>MQARARAFRLKSYADGDLLRELRQFDGAKNASELGPRAFVRDSHRLDAAVEKASKLTDPTFHISQYQLPHPYSFGGGPPNPERPLTAPLISAINKVSQRTRDPVGYRKRAKESIDLGDFTTHDPDTLHPRFLEYVHERTRSVDGPTDDAMRAAQTVFARLWRRKGCKVKARSLSDAQPDNLLAIIKKGSPGEYRSLGAEDRRDPRLIATMSSSLLRYASAGVQVARGRPPPGWVDTTTQVTLTFGKREPKAAKIVDGVRQAPVPRFIFNLSPVNYALASFLHYDISHFLMDNDPTHGPGFGPGRGRARKFMDLVERAFDGRFSTPDGARLIMSDITKWDANMCEALIKYSIDLLEDAVDKSALSPEGLATRGLMYRVARRQLLEKLVEHPAGYFVKLYGCMPSGSFYTSLVNTTGNNLLVIGHAIARAVEETSLTHHGAAELLADAVDGTLISYGDNQLFSEHLFSVLGLAYDPEKH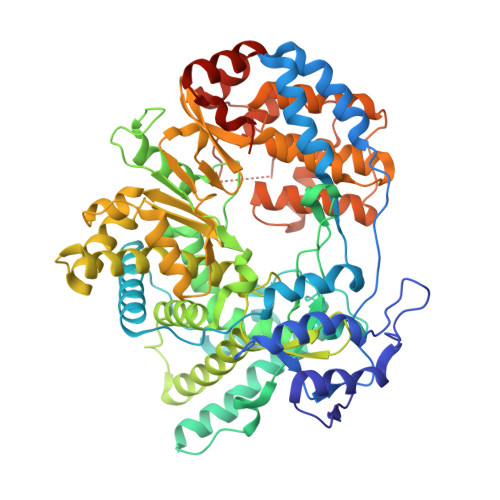AEFLARFGMKLKVDETEVTVKLGRVRFCSRSLVRTPHGLLITRSHNSLFAKLAGRPRHDPVVDKLYVRAMMVDHMGTDPIVYAILNEIDRSLNVSLEAAGLTDAAKKVLEDTAQSMFGNREQDALLAVYRALSETVIDRRALLSLHTPRDGDHDPGRLHTSVSTGMHLFTGELTPAAQWAYECTVEKWCQYLHDTDQEGVMFDGSSSHHHHHH[5x]>[2x]SQAESKEWYHASLTRAQAEHMLMRVPRDG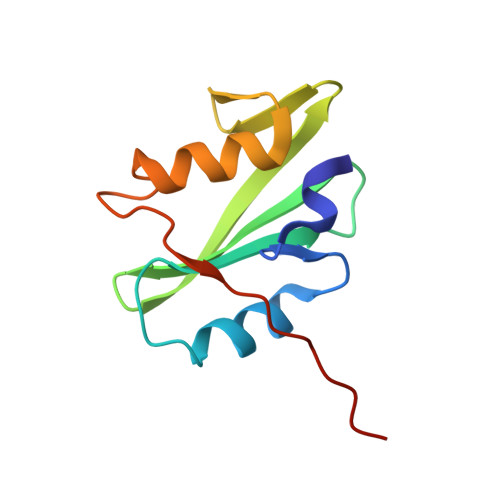AFLVRKRNEPNSYAISFRAEGKIKHCRVQQEGQTVMLGNSEFDSLVDLISYYEKHPLYRKMKLRYPINEEALEKIGT>[4x]MEQSVANLVDMRDVSFTRGNRCIFDNISLTVPRGKIT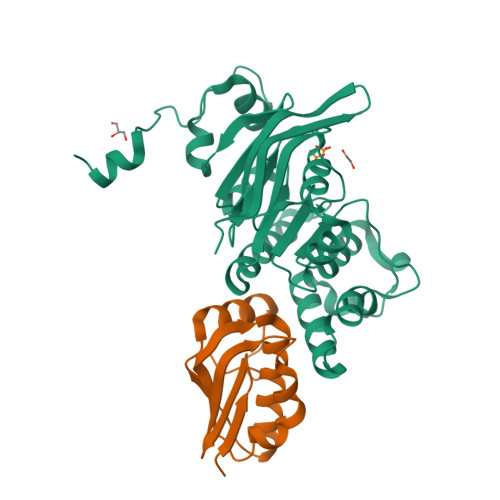AIMGPSGIGKTTLLRLIGGQIAPDHGEILFDGENIPAMSRSRLYTVRKRMSMLFQSGALFTDMNVFDNVAYPLREHTQLPAPLLHSTVMMKLEAVGLRGAAKLMPSELSGGMARRAALARAIALEPDLIMFDEPFVGQDPITMGVLVKLISELNSALGVTCVVVSHDVPEVLSIADHAWILADKKIVAHGSAQALQANPDPRVRQFLDGIADGPVPFRYPAGDYHADLLPGS;>MHHHHHHENLYFQSESLSWMQTGDTLALSGELDQDVLLPLWEMREEAVKGITCIDLSRVSRVDTGGLALLLHLIDLAKKQGNNVTLQGVNDKVYTLAKLYNLPADVLPR[4x]>[2x]MSTFDNKKLRVLCEKELKNSDVGSLGRIVLPKRDAEANLPKLSDKEGIVVQMRDVFSMQSWSFKYKFWSNNKS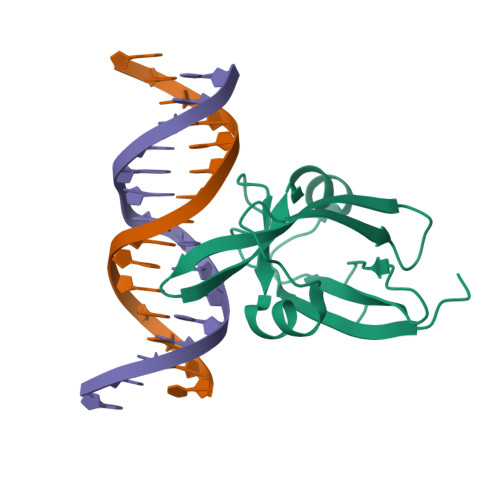RMYVLENTGEFVKQNGAEIGDFLTIYEDESKNLYFAMNGNSGLEHHHHHH> XAT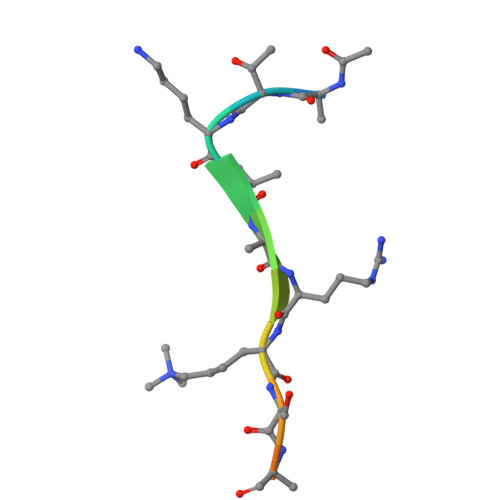KVARKSAPATX> SG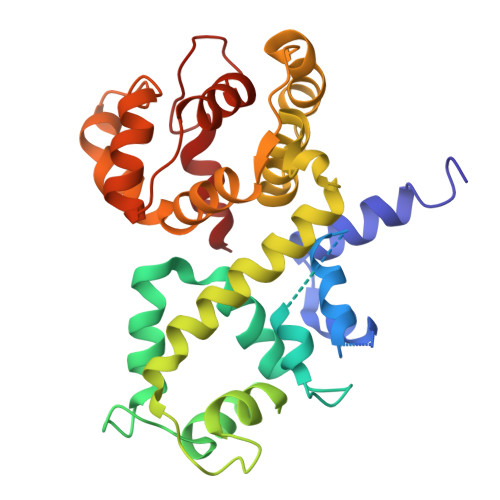FRDRKVMEYENRIRAYSTPDKIFRYFATLKVISEPGEAEVFMTPEDFVRSITPNEKQPEHLGLDQYIIKRFDGKKISQEREKFADEGSIFYTLGECGLISFSDYIFLTTVLSTPQRNFEIAFKMFDLNGDGEVDMEEFEQVQSIIRSQTSMGMRHRDRPTTGNTLKSGLCSALTTYFFGADLKGKLTIKNFLEFQRKLQHDVLKLEFERHDPVDGRITERQFGGMLLAYSGVQSKKLTAMQRQLKKHFKEGKGLTFQEVENFFTFLKNINDVDTALSFYHMAGASLDKVTMQQVARTVAKVELSDHVCDVVFALFDCDGNGELSNKEFVSIMKQRLM>MRGSHHHHHHGSVIFDKRIKDEEDVEKELGLPVLGSIQKFNMTNTRRSTSSLIVHEQPKSPISEKFRGIRSNIMFANPD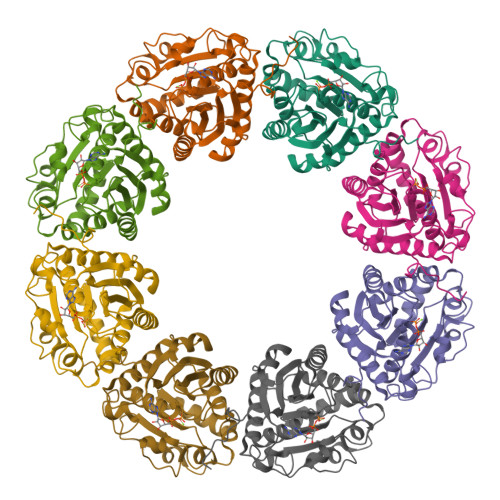SAVQSIVITSEAPGAGMSTIAANLAVAYAQAGYKTLIVDGDMRKPTQHYIFNLPNNEGLSSLLLNWSTYQDSIISTEIEDLDVLTSGPIPPNPSELITSRAFANLYDTLLMNYNFVIIDTPPVNTVTDAQLFSKFTGNVVYVVNSENNNKDEVKKGKELIEATGAKLLGVVLNRMPKDKSASYYAYYGTDES[2x]>SSTILVIHGPNLNLLGKREPEVYGHLTLDNINRQLIAQAEQASITLDTFQSNWEGAIVDRIHQAQTEGVKLIIINPAALTHTSVALRDALLGVAIPFIEVHLSNVHAREAFRHHSYLSDKAIGVICGLGAKG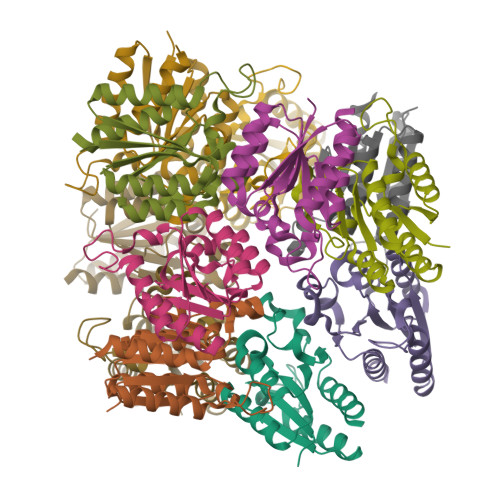YSFALDYAIEKIQ[12x]>PAWTTFRVGLFCGIFIVLNITLVLAAVFKLETDRSIWPLIRIYRGGFLLIEFLFLLGINTYGWRQAGVNHVLIFELNPRSNLSHQHLFEIAGFLGILWCLSLLACFFAPISVIPTYVYPLALYGFMVFFLINPTKTFYYKSRFWLLKLLFRVFTAPFHKVGFADFWLADQLNSLSVILMDLEYMICFYSLELKWDESKGLLPNNSEESGICHKYTYGVRAIVQCIPAWLRFIQCLRRYRDTKRAFPHLVNAGKYSTTFFMVTFAALYSTHKERGHSDTMVFFYLWIVFYIISSCYTLIWDLKMDWGLFDKNAGENTFLREEIVYPQKAYYYCAIIEDV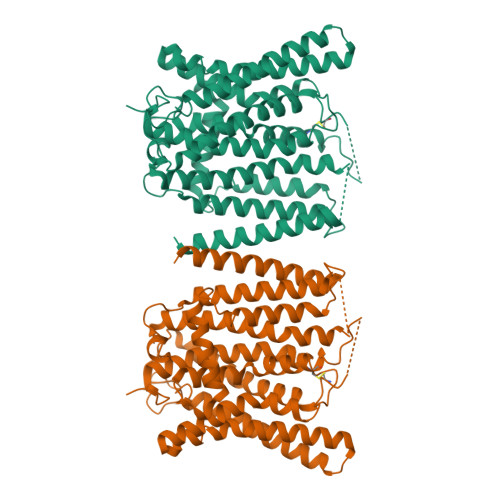ILRFAWTIQISITSTTLLPHSGDIIATVFAPLEVFRRFVWNFFRLENEHLNNCGEFRA[2x]Two host-guest collagen peptides (GPP)4-(GXY)4-(GPP)3, where (GXY)4 sequences are from the α1 and α2 chains of human type I collagen, were recombinantly linked to chains A, B and C (corresponding to α1, α2 and α3 in collagen nomenclature and omitted here to avoid confusion) of the NC2 domain in the following combinations designated as α1Aα1Bα1C (for short 111), α1Aα1Bα2C (112), α1Aα2Bα1C (121), α2Aα1Bα1C (211) and α2Aα2Bα2C (222). Three unique chains form a parallel α-helical right-handed bundle. The most important observation is that the triple-helical chain stagger is entirely determined by the NC2 domain.

All five constructs were screened for crystallization, but only three of them yielded crystals of sufficient quality, crystal structures for 111, 211 and 121 were independently solved using the MAD phasing from selenomethionine derivatives (thereafter designated as 111sm, 211sm and 121sm) to 2.25 Å, 2.10 Å and 1.6 Å, respectively. Whereas the crystal packing for 111sm and 211sm are similar (two trimers per asymmetric unit), it differs from that for 121nat or 121sm (one trimer per asymmetric unit). Overall superimposition of all trimers showed some drastic deviations. The most deviated pair is the first trimer (chains A, B, C in the asymmetric unit) of 121sm versus the second trimer (chains D, E, F) of 111sm (r.m.s.d. of 3.01 Å). On the other hand, superimposition within the NC2 domain demonstrated high identity of the trimerization domain and adjacent residues within the triple-helical portion. Most of deviations observed for overall superimposition of trimers are attributed to distal flexibility of the triple helical fragments caused by crystal packing (Fig. 2A vs B). Namely, a triple helical chain linked to chain B of the NC2 domain is always in the leading position, the one linked to A is in the middle, and the third one linked to C is in the trailing position. Despite the variations of composition (homo-trimeric for 111) and stagger (121 or 211) that might not represent a native stagger, the regions of sequences derived from type I collagen are well structured. Crystal structures of 111, 121 and 211 constructs demonstrated that a staggering order can be manipulated at least for short native collagenous sequences, meaning that such sequences are rather adaptive to various abnormal conformations.

>GSGPPGPPGPPGPPGARGQAGVMGFPGPPGPPGPPGRAPTDQHIKQVCMRVIQEHFAEMAASLKRPDSGAT[2x];>[2x]GSGPPGPPGPPGPPGARGQAGVMGFPGPPGPPGPPGRDATDQHIVDVALKMLQEQLAEVAVSAKREALGAV;>GSGPPGPPGPPGPPGARGQAGVMGFPGPPGPPGPPGKEASEQRIRELCGGMISEQIAQLAAHLRKPLAPGSI[2x]> SNNWAVAPGRTATGRPILAGDPHRVFEIPGFYAQHHLACDRFDMIGLTVPGVPG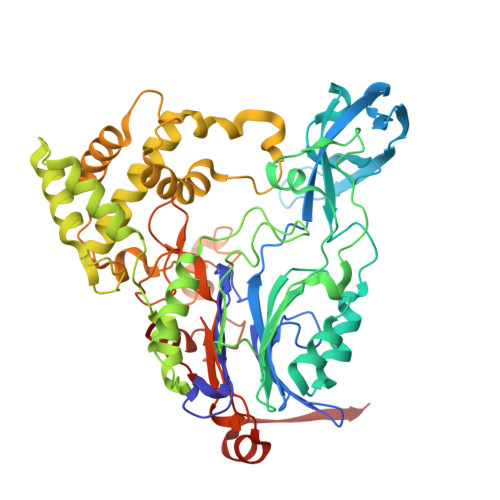FPSFAHNGKVAYCVTSAFMDIHDLYLEQFAGEGRTARFGNDFEPVAWSRDRIAVRGGADREFDIVETRHGPVIAGDPRDGAALTLRSVQFAETDLSFDCLTRMPGASTVAQLYDATRGWGLIDHNLVAGDVAGSIGHLVRARVPSRPRENGWLPVPGWSGEHEWRGWIPHEAMPRVIDPPGGIIVTANNRVVADDHPDYLCTDCHPPYRAERIMKRLVANPAFAVDDAAAIHADTLSPHVGLLRRRLEALGARDDSAAEGLRQMLVAWDGRMDAASEVASAYNAFRRALTRLVTDRSGLEQAISHPFAAVAPGVSPQGQVWWAVPTLLRDDDAGMLKGWSWDQALSEALSVASQNLTGRSWGEEHRPRFTHPLATQFPAWAGLLNPASRPIGGDGDTVLANGLVPSAGPQATYGALSRYVFDVGNWDNSRWVVFHGASGHPASAHYADQNAPWSDCAMVPMLYSWDRIAAEAVTSQELVPALEHHHHHH>[4x]GPGSSLSRFRGCLAGALLGDCVGSFYAAHDTVDLTSVLRHVQSLEPDPGTPGSERTEALYYTDDTAMARALVQSLLAKEAFDEVDMAHRFAQEYKKDPDRGYGAGVVT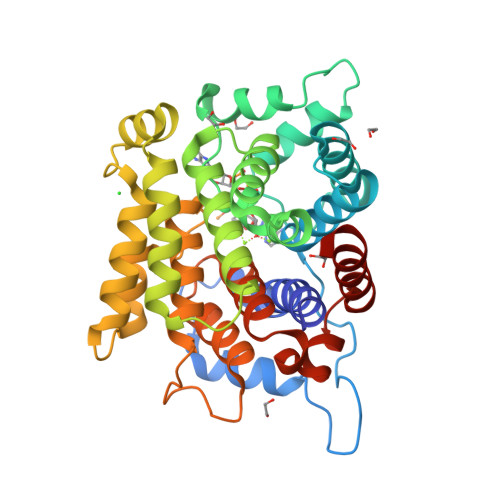VFKKLLNPKCRDVFEPARAQFNGKGSYGNGGAMRVAGISLAYSSVQDVQKFARLSAQLTHASSLGYNGAILQALAVHLALQGESSSEHFLKQLLGHMEDLEGDAQSVLDARELGMEERPYSSRLKKIGELLDQASVTREEVVSELGNGIAAFESVPTAIYCFLRCMEPDPEIPSAFNSLQRTLIYSISLGGDTDTIATMAGAIAGAYYGMDQVPESWQQSCEGYEETDILAQSLHRVFQKS>[16x]KKGYEVLRDPHLNKGMAFTLEERQQLNIHGLLPPCFLGQDAQVYSILKNFERLTSDLDRYILLMSLQDRNEKLFYKVLTSDIERFMPIVYTPTVGLACQHYGLAFRRPRGLFITIHDRGHIATMLQSWPESVIKAIVVTDGERILGLGDLGCYGMGIPVGKLALYTACGGVKPHQCLPVMLDVGTDNETLLKDPLYIGLRHKRIRGQAYDDLLDEFMEAVTSRYGMNCLIQFEDFANANAFRLLHKYRNKYCTFNDDIQGTASVAVAGLLAALRITKNRLSDHTVLFQGAGEAALGIANLIVMAMQKEGVSKEEAIKRIWMVDSKGLIVKGRASLTPEKEHFAHEHCE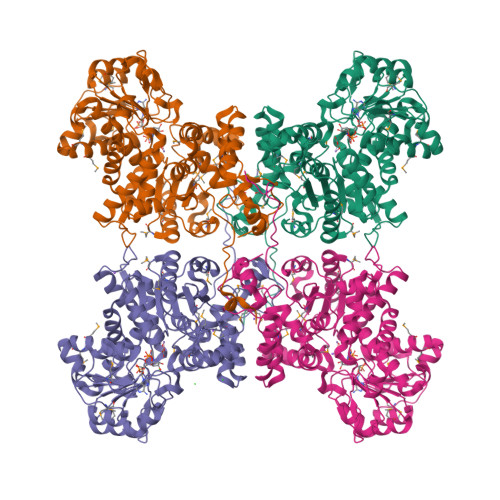MKNLEDIVKDIKPTVLIGVAAIGGAFTQQILQDMAAFNKRPIIFALSNPTSKAECTAEQLYKYTEGRGIFASGSPFDPVTLPSGQTLYPGQGNNSYVFPGVALGVISCGLKHIGDDVFLTTAEVIAQEVSEENLQEGRLYPPLVTIQQVSLKIAVRIAKEAYRNNTASTYPQPEDLEAFIRSQVYSTDYNCFVADSYTWPEEAMKVK> MSTLEQTIGNTPLVKLQRMGPDNGSEVWLKLEGNNPAGSVKDRAALSMIVEAEKRGEIKPGDVLIEATSGNTGIALAMIAALKGYRMKLLMPDNMSQERRAAMRAYGAELILVTKEQGMEGARDLALEMANRGEGKLLDQFNNPDNPYAHYTTTGPEIWQQTGGRITHFVSSMGTTGTITGVSRFMREQSKPVTIVGLQPEEGSSIPGIRRWPTEYLPGIFNASLVDEVLDIHQRDAENTMRELAVREGIFCGVSSGGAVAGALRV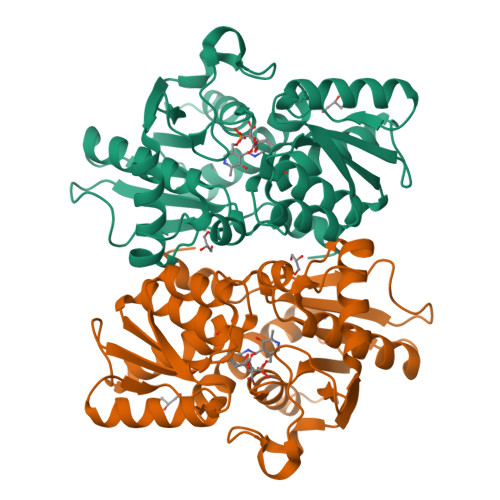AAANPDAVVVAIICDRGDRYLSTGVFGEEHFSQGAGI> SGSGLKELLKELNKAIAS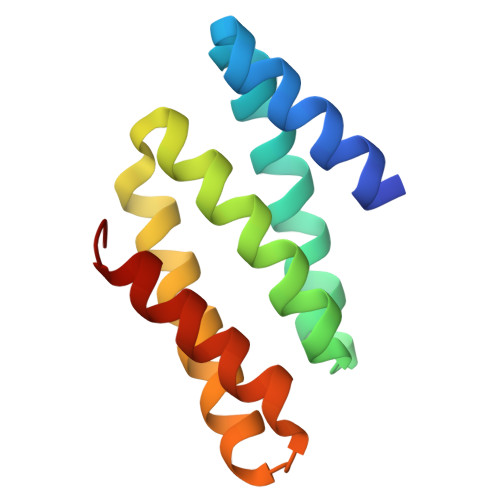GDTETVRRILEELLELLKEAFEKGDYDLAISIASMAVKAASYIGDTETLKELLEILKKIKEKLKKEGDEAALKAVERNIKVVEKVA> MSSTIFYRFKSQRNTSRILFDGTGLTVFDLKREIIQENKLGDGTDFQLKIYNPDTEEEYDDDAFV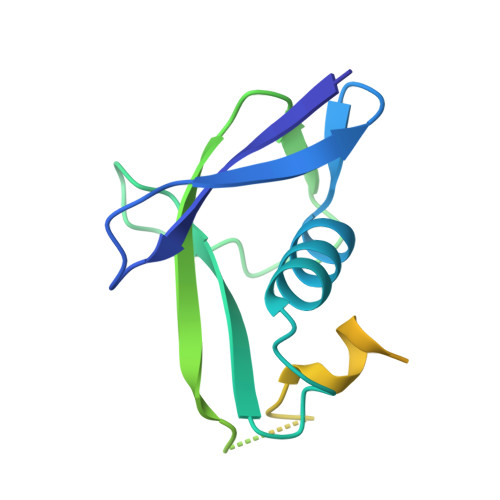IPRSTSVIVKRSPAIKSFSVHSRLKGNVGAAAKGNATRYVTGRPRVLQKRQHTATTTANVSGTTEEERIASMFATQENQWEQTQEEMSAATPVFF>SNAMTDAVLE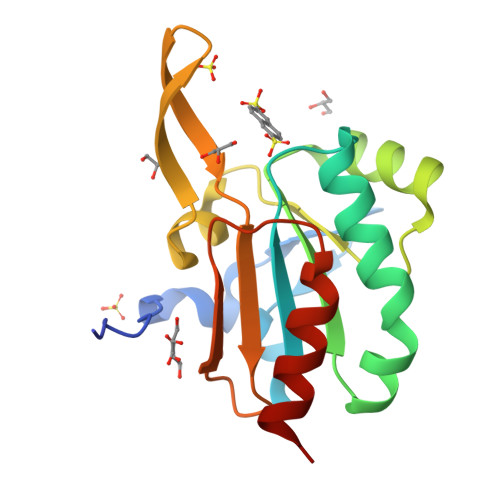LPAATFDLPLSLSGGTQTTLRAHAGHWLVIYFYPKDSTPGATTEGLDFNALLPEFDKAGAKILGVSRDSVKSHDNFCAKQGFAFPLVSDGDEALCRAFDVIKEKNMYGKQVLGIERSTFLLSPEGQVVQAWRKVKVAGHADAVLAALKAHAKQ[2x]>[6x]MVTYTTLLDKPISESAPRKAPEPLLRE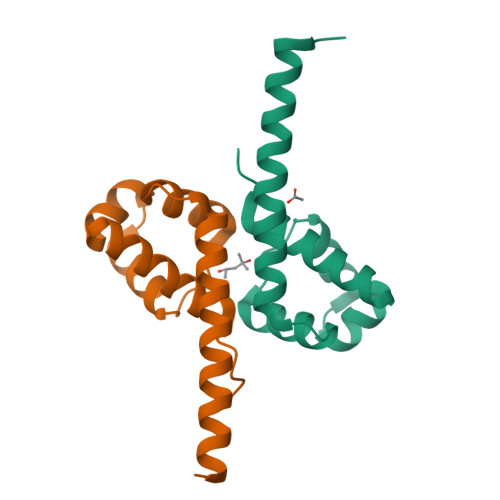ALGAALRSFRADKGVTLRELAEASRVSPGYLSELERGRKEVSSELLASVCHALGASVADVLIEAAGSMALQAAQEDLARVLEWSHPQFEK>MAHHHHHHMIYRTEHDTMGEVKVPVDKFWGAQTERSRNNFKIGPEASMPHEIIEAFAYLKKAAAYANTDLRVLPSDKRDMISQVCDEILEGKLFDQFPLVIWQTGSGTQSNMNINEVISNKAHVNNGGQLGEKSEVHPNDDVNKSQSSNDTYPTAMHIAAYKKVVEHTIPAVETLKNTLKAKSEAFKNIVKIGRTHLMDATPLTLGQEFSGYVAQLEFGLKALKNTLPHLAELALGGTAVGTGLNTPQGYDVKVAEYIAKFTGLPFITAENKFEALAAHDAIVESHGALKQLAVSLFKIAQDIRM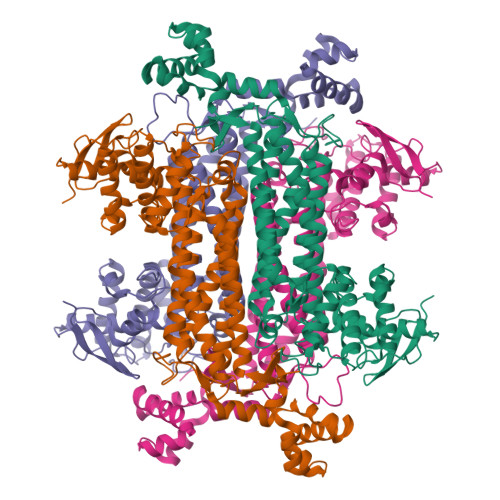LASGPRSGIGEIHIPENEPGSSIMPGKVNPTQNEAMTMVCAQVLGNDTTISFAGTQGNYELNVFKPVMAYNFLQSAQLIADACISFNDHCAVGIEPNEPRIKELVDKSLMLVTALNTHIGYENAAKIAKTAHKNGTTLKEEAINLGLVTAEQFDEWVKPEDMVGSLK[4x]>[3x]CTVGPDYRTPDTAAAKIDATASKPYDRSRFESLWWKQFDDPTLNQLVEQSLSGNRDLRVAFARLRAARALRDDVANDRFPVVTSRASADIGKGQQPGVTEDRVNSERYDLGLDSAWELDLFGRIRRQLESSDALSEAAEADLQQLQVSLIAELVDAYGQLRGAQLREKIALS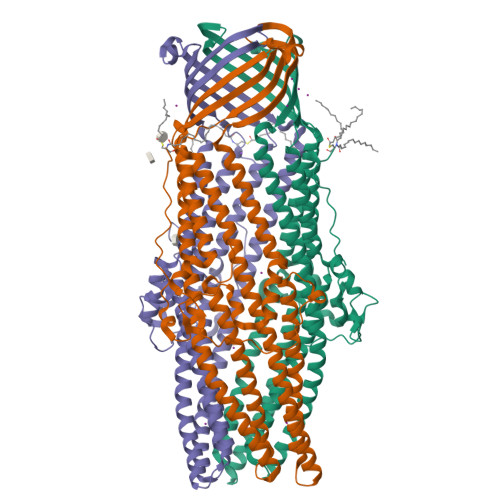NLENQKESRQLTEQLRDAGVGAELDVLRADARLAATAASVPQLQAEAERARHRIATLLGQRPEELTVDLSPRDLPAITKALPIGDPGELLRRRPDIRAAERRLAASTADVGVATADLFPRVSLSGFLGFTAGRGSQIGSSAARAWSVGPSISWAAFDLGSVRARLRGAKADADAALASYEQQVLLALEESANAFSDYGKRQERLVSLVRQSEASRAAAQQAAIRYREGTTDFLVLLDAEREQLSAEDAQAQAEVELYRGIVAIYRSLGGGWQPSAHHHHHH>[3x]MGKSLSHLPLHSSKEDAYDGVT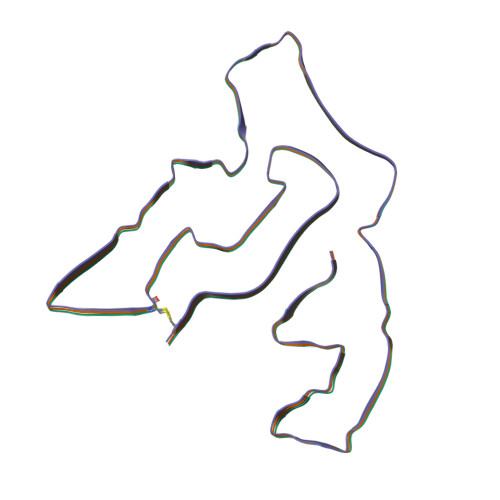SENMRNGLVNSEVHNEDGRNGDVSQFPYVEFTGRDSVTCPTCQGTGRIPRGQENQLVALIPYSDQRLRPRRTKLYVMASVFVCLLLSGLAVFFLFPRSIDVKYIGVKSAYVSYDVQKRTIYLNITNTLNITNNNYYSVEVENITAQVQFSKTVIGKARLNNISIIGPLDMKQIDYTVPTVIAEEMSYMYDFCTLISIKVHNIVLMMQVTVTTTYFGHSEQISQERYQYVDCGRNTTYQLGQSEYLNVLQPQQ>[2x]MRGETLKLKKDKRREAIRQQIDSNPFITDHELSDLFQVSIQTIRLDRTYLNIPELRKRIKLVAEKNYD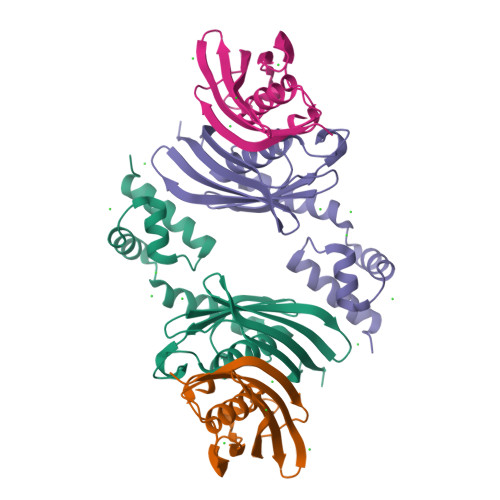QISSIEEQEFIGDLIQVNPNVKAQSILDITSDSVFHKTGIARGHVLFAQANSLCVALIKQPTVLTHESSIQFIEKVKLNDTVRAEARVVNQTAKHYYVEVKSYVKHTLVFKGNFKMFYDKRG>GSHMAAVQKLFPYTPRAPIRQGIYSQAVVVDRTMYISGQLGLDVASGKLVEGGVQAQARQALVNMGEILKAAGCGYDNVVKTTVLLADMNDFVNVNDVYKTFFSKNFPARAAYQVVALPRGGLVEIEAVAVLGPISES[6x]

The term Rid (reactive intermediate deaminase) refers to the hydrolytic deamination of highly reactive and labile enamines/imines to α-ketoacid and ammonia, a reaction that would be otherwise relatively slow if left to occur spontaneously. In the present study, we identified two functionally active RidA genes in the salmon genome, here named ridA-1 and ridA-2, and we performed an extensive biochemical and structural characterization of their products (SsRidA-1 and SsRidA-2). In order to better understand the structural bases of the observed differences in terms of protein stability and of enzymatic activity, the crystal structures of SsRidA-1 and SsRidA-2 were determined at 1.05 Å and at 1.36 Å resolutions, respectively. Monomeric SsRidA-1 and SsRidA-2 share the chorismate mutase-like fold common to all the members of the YjgF/YER057c/UK114 superfamily: monomers fold in a single compact domain of one six-stranded β-sheet packed against two α-helices.

The two SsRidA-2 trimers are virtually identical (r.m.s.d. values 0.45 Å/380 Cα) and also SsRidA-2 monomers are all well superposable (r.m.s.d. values in the 0.15–0.26 Å range over the whole Cα chain). However, SsRidA-2 is the only ortholog with a Pro residue in position 9 in place of Ile or Val in the other analysed sequences. Residue 9 is part of strand β1 and a substitution of Val or Ile, which are highly compatible with a β-structure, with Pro, a β-breaker, results in a shorter and less regular β1 strand in SsRidA-2 compared to SsRidA-1. In SsRidA-2 this intermolecular two-strand β-sheet is not present and both regions are partially disordered in the structure. Secondly, the shortening of β1strand by Pro9 reduces the H-bond network in the central β sheet likely decreasing the stability of the monomeric fold. Crucially, residues 16–18 are typically small and hydrophobic in RidA primary structures, while Arg and Gln are present in position 17 and 18, respectively, in SsRidA-2. This confers very different chemical properties to SsRidA-2 binding pocket compared to SsRidA-1. On the other hand, SsRidA-2 has a positive charge in position 17 and, under our experimental conditions, showed a strong preference for the IA derived from L-Glu, while the lack of activity on the IA derived from L-Asp cannot be explained. On the other hand, SsRidA-2 showed a more canonical denaturation curve revealing a Tm of 65 °C.> SMHSDLTFCEIILMEMESHDAAWPFLEPVNPRLVSGYRRIIKNPMDFSTMRERLLRGGYTSSEEFAADALLVFDNCQTFNEDDSEVGKAGHIMRRFFESRWEEFY

BAZ2A is an epigenetic regulator affecting transcription of ribosomal RNA. It is overexpressed in aggressive and recurrent prostate cancer, promoting cellular migration. BAZ2A, however, features a shallow pocket, making it one of the least druggable bromodomains. Here, we describe a structure-based fragment-growing campaign for the identification of ligands of the BAZ2A bromodomain.

The binding mode of compound 13 is unexpected. It runs parallel to the end of the αB helix, similarly to the Kac residue of acetylated peptides, instead of facing the WPF shelf of the ZA loop. Consequently, the charged piperidine is not directed toward Glu1820 but rather exposed to the solvent. The amide of compound 13 does not reciprocally interact with the side chain of Asn1823, unusually placing the amide nitrogen in the small pocket reserved for the KAc methyl group in physiological ligands. While the amide oxygen interacts with both Asn1823 and Tyr1830 (W1-bridged), the amide nitrogen establishes H-bonds to main-chain oxygens of Pro1817 and Val1865, the latter mediated by a water molecule (W3).> MPRGGRPQKVAAHITGITRRSNSALIPISKDGKTLGQKIESWESSRKGHSFLNHVLFRNGELVIEQEGLYYIYSQTYFRFQEAEDASKMVSKDKVRTKQLVQYIYKYTSYPDPIVLMKSARNSCWSRDAEYGLYSIYQGGLFELKKNDRIFVSVTNEHLMDLDQEASFFGAFLIN

TRAIL (TNF-related apoptosis-inducing ligand) is a potent inducer of tumor cell apoptosis through TRAIL receptors. TNF superfamily ligands are expressed as type II transmembrane proteins and form homotrimers through their extracellular domains. TRAIL is known to bind five members of the TNF receptor superfamily. TRAIL binds HS with high affinity (KD = 73 nM) and HS induces TRAIL to form higher-order oligomers.

We determined the crystal structure of soluble mTRAIL to better compare to hTRAIL and understand the biophysical characterization of HS and mTRAIL interactions. Though a HS 12mer was present in the crystallization conditions, the oligosaccharide was not visible in the electron density. Similar to hTRAIL, mTRAIL exists as a trimer composed of three β-scaffold core protomers with one protomer comprising the asymmetric unit. A zinc ion, critical for activity, is located on the threefold axis bound by cysteine 240 from each protomer and a chloride ion. A major difference between TRAIL and other TNF family members is an insertion of ~12–16 residues between β-strands A and Aʺ known as the A-Aʺ loop (or AAʺ loop, Figure 3A; Cha et al., 1999). The N-terminal β-strand A of mTRAIL is found sandwiched between β-stands H and Aʺ of the neighboring protomer’s central β-scaffold core, a pattern repeated for each protomer. Clear electron density can be traced between this strand and β-strand Aʺ confirming the swapping of the N-terminal strand between the protomers. Interestingly, this swap has not been reported in other structures of TRAIL or TNF family members. To explicitly determine the HS-binding site of TRAIL, we performed site-directed mutagenesis of seven conserved lysine and arginine residues on mTRAIL, some of which (Arg119, Arg122, and Lys125) cluster (in triplicate) near the ‘top’ of the trimer and likely form the HS-binding site. Interestingly, these three residues are located at the N-terminus of the soluble TRAIL, which likely adopts a random coil structure because it was not visible in the crystal structure of soluble TRAIL.>MNNFGNEEFDCHFLDEGFTAKDILDQKINEVSSSDDKDAFYVADLGDILKKHLRWLKALPRVTPFYAVKCNDSKAIVKTLAATGTGFDCASKTEIQLVQSLGVPPERIIYANPCKQVSQIKYAANNGVQMMTFDSEVELMKVARAHPKAKLVLRIATDDSKAVCRLSVKFGATLRTSRLLLERAKELNIDVVGVSFHVGSGCTDPETFVQAISDARCVFDMGAEVGFSMYLLDIGGGFPGSEDVKLKFEEITGVINPALDKYFPSDSGVRIIAEPGRYYVASAFTLAVNIIAKKIVLKEQTGSDDEDESSEQTFMYYVNDGVYGSFNCILYDHAHVKPLLQKRPKPDEKYYSSSIWGPTCDGLDRIVERCDLPEMHVGDWMLFENMGAYTVAAASTFNGFQRPTIYYVMSGPAWQLMQQFQN[2x]

Ornithine decarboxylase (ODC) is a pyridoxal phosphate (PLP)-dependent enzyme that catalyzes the conversion of ornithine to putrescine, a rate-limiting first step for the tightly regulated biosynthesis of polyamines (putrescine, spermidine, spermine).1−3 At the molecular level, positively charged polyamines interact with negatively charged RNA, DNA, and phospholipids, thereby directly contributing to chromatin biology. The ODC enzyme is a homodimer, with the dimer interface forming its catalytic site from residues from both monomers. We report two X-ray structures of ODC complexed with new ODC inhibitors, computational docking, molecular dynamics, and binding free energy calculations to validate the experimental models. The X-ray structures reveal that covalent adducts with pyridoxal phosphate (PLP) are formed in the active site of the human ODC enzyme, as verified by their preparation and enzymatic testing.

We then turned our attention to the inclusion of the 5-membered pyrrolidine analogs. Compounds 10, 10-R and 10-S had ODC IC50 values of 0.36, 0.21, and 0.10 μM, respectively. As before, it is anticipated that the PLP adducts are formed in the active site and are the true inhibitors. To help verify, we have also prepared 10-R-PLP and 10-S-PLP and found that they both demonstrate inhibition of ODC enzymatic activity, with IC50 values of 0.16 and 0.03 μM, respectively. The activity still favors, as observed for 10-R and -S, the S-enantiomer with 8-fold relative activity. In each case, as we saw with APA, the adducts 10-R-PLP (2.9 Å resolution) and 10-S-PLP (2.0 Å resolution) were formed, forming trans-oximes with PLP. The lipophilic cyclic pyrrolidines of 10-R-PLP and -S-PLP, form strong lipophilic interactions with Tyr389 and weaker lipophilic interactions with Phe397, the pyrrolidine rings orientated in an orthogonal manner relative to each other. The basic pyrrolidine amine of each makes a H-bonding interaction with Asp331. Although the structure associated with 10-R-PLP is of lower resolution and does not include water molecules in the structure, a well-defined H-bond network of direct interactions is available, which explains the similarity of activities observed. While there are some small differences between each structure, both networks appear to be equally strong.Ktr4p is a member of the Kre2/Mnt1 family of glycosyltransferases. Ktr4p, as the other members of the Kre2/Mnt1 family, is a type II membrane protein with a short N-terminal cytosolic tail and a large lumenal catalytic domain of 40 kDa, which is separated from the membrane by a stalk domain of 11 kDa. Ktr4p, with its large central β-sheet, belongs to the GT-A fold class of glycosyltransferases. We used GDP-mannose as the sugar donor, and tested mannose, α-1,2-mannobiose and methyl-α-mannoside as potential acceptors; in the case of both donor and acceptor this was based on suggestions from sequence identity. Our results, shown in Fig 4, confirm that Ktr4p is an active mannosyltransferase enzyme.

We have formed the complex of Ktr4p and GDP and Mn2+ by soaking crystals of the apo-form, and solved the structure of this complex to 1.9 Å resolution. Both ligands bind in the previously described active-site cleft, which is situated on the surface of the protein, as seen in Fig 2. The most noticeable difference, apart from the GDP itself, is the presence of a Mn2+ ion bound in the active site of each monomer in the complex. The Mn2+ ion in the active site is hexahedrally coordinated. The metal ion interacts with the OE1 of Glu-262 at a distance of 2.2 Å, the NE2 of His-411 (2.4 Å), water molecules 1 and 2 (both at 2.4 Å distance), as well as the O1 of the α- (2.3 Å) and the O1 of the β-phosphate (2.2 Å). O1 of the β-phosphate interacts with the OH of Tyr-229 at a distance of 2.7 Å, and O2 of the β-phosphate interacts with the OH of Tyr-235 at a distance of 2.7 Å. The guanine moiety of the GDP makes hydrogen bonds to three residues of the enzyme via its nitrogen atoms; N1 interacts with OD1 of Asp-173 at 2.7 Å distance, while N2 interacts with the same atom (3.2 Å distance), OD1 of Asn-172 (2.9 Å) and the main chain O of Val-141 (3.0 Å). Only slight changes in sidechain conformation can be observed upon ligand binding in the active site, most notably the position of Arg-142 changes upon ligand binding to free space for the nucleotide base and interact with it via a stacking interaction, meaning the gross structure of the active site pocket is preformed in the proteins apo-state despite the absence of the Mn2+ ion. In the complex structure Glu-262 is coordinating the active site Mn2+ ion via its OE1 atom, while Asn-264 is on the surface of the monomer and is indirectly interacting with the second chain of the ‘dimer’ via two water molecules. Despite extensive efforts to produce a structure of Ktr4p in complex with GDP-mannose, both by co-crystallisation and by soaking native crystals with GDP-mannose, we have not been able to observe the non-hydrolysed state of the ligand, but only the GDP moiety.

>[2x]SMNENYLQAVKDSAKSQYASLRESYKSITGKTESADELPDHDAEVLDSIMDRLHEPLYEKDTFDPNEVLAENKQLYEEFLLQEISEPKVDNLVRSGDPLAGKAKGTILSLVRNSDLEDIISSIQQLEEEYNKNFGYPYTFLNDEEFTDEFKDGIKSILPKDRVVEFGTIGPDNWNMPDSIDRERYDQEMDKMSKENIQYAEVESYHNMCRFYSKEFYHHPLLSKYKYVWRLEPNVNFYCKINYDVFQFMNKNDKIYGFVLNLYDSPQTIETLWTSTMDFVEEHPNYLNVNGAFAWLKDNSQNPKNYDYTQGYSTCHFWTNFEIVDLDFLRSEPYEKYMQYLEEKGGFYYERWGDAPVRSLALALFADKSSIHWFRDIGYHHTPYTNCPTCPADSDRCNGNCVPGKFTPWSDLDNQNCQATWIRHSMSEEELEMY> DERFYAEHLMPTLQGLLDPESAHRLAVRFTSLGLLPRARFQDSDMLEVRVLGHKFRNPVGIAAGFDKHGEAVDGLYKMGFGFVEIGSVTPKPQEGNPRPRVFRLPEDQAVINR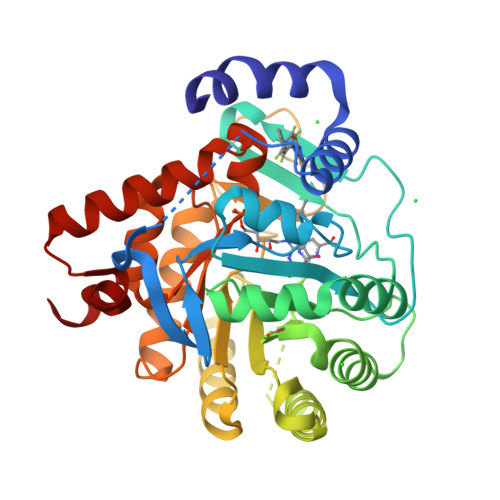YGFNSHGLSVVEHRLRARQQKQAKLTEDGLPLGVNLGKNKTSVDAAEDYAEGVRVLGPLADYLVVNVSSPNTAGLRSLQGKAELRRLLTKVLQERDGLRRVHRPAVLVKIAPDLTSQDKEDIASVVKELGIDGLIVTNTTVSRPAGLQGALRSETGGLSGKPLRDLSTQTIREMYALTQGRVPIIGVGGVSSGQDALEKIRAGASLVQLYTALTFWGPPVVGKVKRELEALLKEQGFGGVTDAIGADHRR>[2x]MGSSHHHHHHSQDPMEMTSAFTLNVRLDNIAVITIDVPGEKMNTLKAEFASQVRAIIKQLRENKELRGVVFVSAKPDNFIAGADINMIGNCKTAQEAEALARQGQQL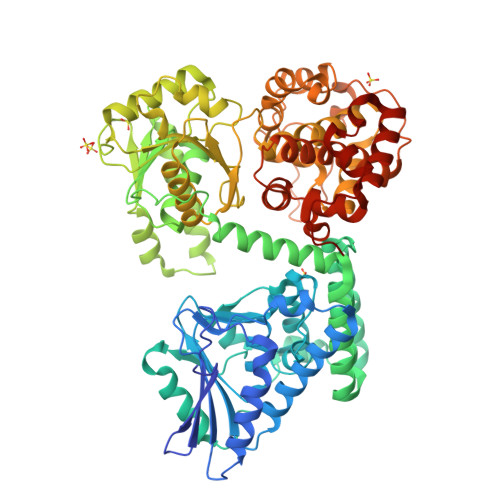MAEIHALPIQVIAAIHGACLGGGLELALACHGRVCTDDPKTVLGLPEVQLGLLPGSGGTQRLPRLIGVSTALEMILTGKQLRAKQALKLGLVDDVVPHSILLEAAVELAKKERPSSRPLPVRERILAGPLGRALLFKMVGKKTEHKTQGNYPATERILEVVETGLAQGTSSGYDAEARAFGELAMTPQSQALRSIFFASTDVKKDPGSDAPPAPLNSVGILGGGLMGGGIAYVTACKAGIPVRIKDINPQGINHALKYSWDQLEGKVRRRHLKASERDKQLALISGTTDYRGFAHRDLIIEAVFENLELKQQMVAEVEQNCAAHTIFASNTSSLPIGDIAAHATRPEQVIGLHFFSPVEKMPLVEIIPHAGTSAQTIATTVKLAKKQGKTPIVVRDKAGFYVNRILAPYINEAIRMLTQGERVEHIDAALVKFGFPVGPIQLLDEVGIDTGTKIIPVLEAAYGERFSAPANVVSSILNDDRKGRKNGRGFYLYGQKGRKSKKQVDPAIYPLIGTQGQGRISAPQVAERCVMLMLNEAVRCVDEQVIRSVRDGDIGAVFGIGFPPFLGGPFRYIDSLGAGEVVAIMQRLATQYGSRFTPCERLVEMGARGESFWKTTATDLQ> GSSAPRFLTRPKAFVVSVGKDATLSCQIVGNPTPQVSWEKDQQPVAAGARFRLAQDGDLYRLTILDLALGDSGQYVCRARNAIGEAFAAV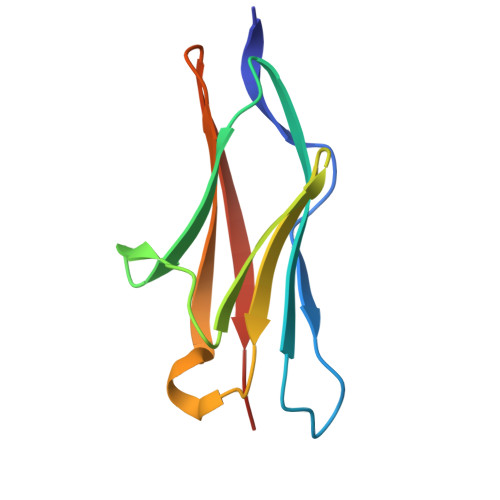GLQVDAEA>MHNLQQLLPTRSLIWIFSFLTSISIWCTVAHAETEGRVQHFTGYIEDGRGIFYSLPDMKQGDIIYASMQNTGGNLDPLVGIMAEEIDPAVSLGQVLEKALASENDLISELTAVADRIFLGWDDDGGKGYSASLEFTIPRDGTYHIFAGSTITNQRLDKFQPTY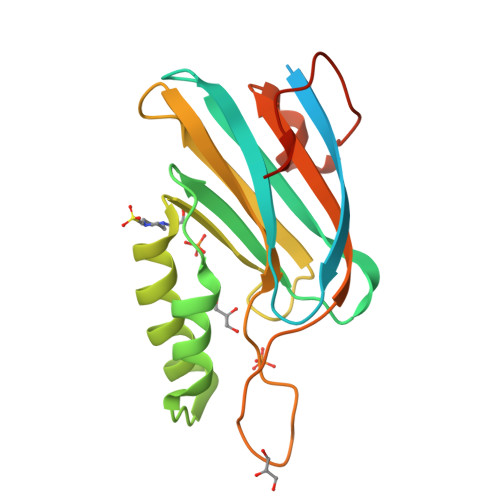TTGSFQLILGLNAPQVISGEGEPEGEVFASLASLEIKPE[2x]> MSILTETVLPGIVQITMNRPERKNALDRACYQGLIDAITAAEADPDIRAMVLTGAGGCFTSGNDIKDFAGAAETGPRVAMDYLGVLSTAKKPIVAAVEGFAVGIGTTMLLHCDLAFAGKGASFRMPFV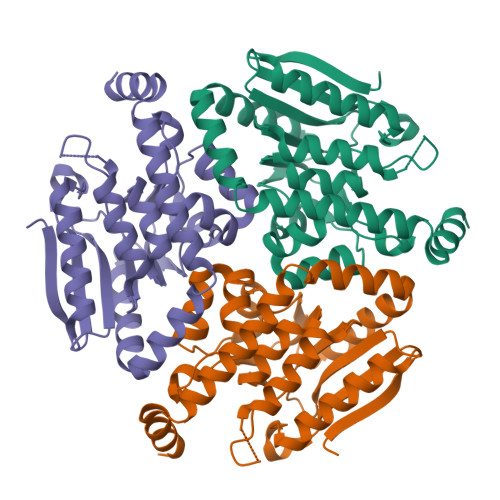ALGLSPEGASSYLLPLIAGSKRAAELLMLGEAFGPEIAHEAGLLNAVTPEGGALALAIEKARALAALPPQSVALTKMLLKRAQAPAVAETIATEGRLFGERLLSAEAQAAFAAFLKR> SKIVKIIGREIIDSRGNPTVEAEVHLEGGFVGMAAAPSGASTGSREALELRDGDKSRFLGKGVTKAVAAVNGPIAQALIGKDAKDQAGIDKIMIDLDGTENKSKFGANAILAVSLANAKAAAAAKGMPLYEHIAELNGTPGKYSMPVPMMNIINGGEHADNNVDIQEFMIQPVGAKTVKEAIRMGSEVFHHLAKVLKAKGMNTAVGDEGGYAPNLGSNAEALAVIAEAVKAAGYELGKDITLAMDCAASEFYKDGKYVLAGEGNKAFTSEEFTHFLEELTKQYPIVSIEDGLDE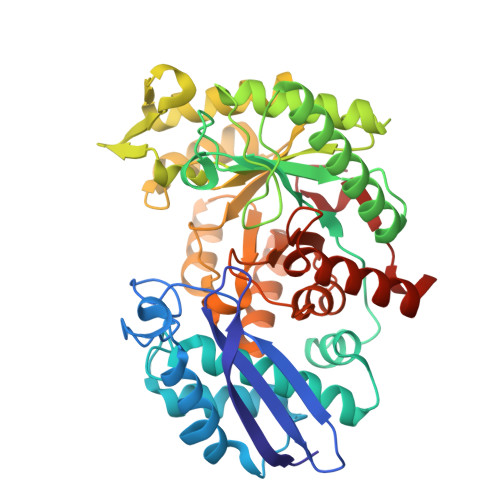SDWDGFAYQTKVLGDKIQLVGDDLFVTNTKILKEGIEKGIANSILIKFNQIGSLTETLAAIKMAKDAGYTAVISHRSGETEDATIADLAVGTAAGQIKTGSMSRSDRVAKYNQLIRIEEALGEKAPYNGRKEIKGQA>MESRVTPVAVIGMGCRLPGGINSPDKLWESLLRGDDLVTEIPPDRWDADDYYDPEPGVPGRSVSRWGGFLDDVAGFDAEFFGISEREATSIDPQQRLLLETSWEAIEHAGLDPASLAGSSTAVFTGLTHEDYLVLTTTAGGLASPYVVTGLNNSVASGRIAHTLGLHGPAMTFDTACSSGLMAVHLACRSLHDGEADLALAGGCAVLLEPHASVAASAQGMLSSTGRCHSFDADADGFVRSEGCAMVLLKRLPDALRDGNRIFAVVRGTATNQDGRTETLTMPSEDAQVAVYRAALAAAGVQPETVGVVEAHGTGTPIGDPIEYRSLARVYGAGTPCALGSAKSNMGHSTASAGTVGLIKAILSLRHGVVPPLLHFNRLPDELSDVETGLFVPQAVTPWPNGNDHTPKRVAVSSFGMSGTNVHAIVEEAPAEASAPESSPGDAEVGPRLFMLSSTSSDALRQTARQLATWVEEHQDCVAASDLAYTLARGRAHRPVRTAVVAANLPELVEGLREVADGDALYDAAVGHGDRGPVWVFSGQGSQWAAMGTQLLASEPVFAATIAKLEPVIAAESGFSVTEAITAQQTVTGIDKVQPAVFAVQVALAATMEQTYGVRPGAVVGHSMGESAAAVVAGALSLEDAARVICRRSKLMTRIAGAGAMGSVELPAKQVNSELMARGIDDVVVSVVASPQSTVIGGTSDTVRDLIARWEQRDVMAREVAVDVASHSPQVDPILDDLAAALADIAPMTPKVPYYSATLFDPREQPVCDGAYWVDNLRNTVQFAAAVQAAMEDGYRVFAELSPHPLLTHAVEQTGRSLDMSVAALAGMRREQPLPHGLRGLLTELHRAGAALDYSALYPAGRLVDAPLPAWTHARLFIDDDGQEQRAQGACTITVHPLLGSHVRLTEEPERHVWQGDVGTSVLSWLSDHQVHNVAALPGAAYCEMALAAAAEVFGEAAEVRDITFEQMLLLDEQTPIDAVASIDAPGVVNFTVETNRDGETTRHATAALRAAEDDCPPPGYDITALLQAHPHAVNGTAMRESFAERGVTLGAAFGGLTTAHTAEAGAATVLAEVALPASIRFQQGAYRIHPALLDACFQSVGAGVQAGTATGGLLLPLGVRSLRAYGPTRNARYCYTRLTKAFNDGTRGGEADLDVLDEHGTVLLAVRGLRMGTGTSERDERDRLVSERLLTLGWQQRALPEVGDGEAGSWLLIDTSNAVDTPDMLASTLTDALKSHGPQGTECASLSWSVQDTPPNDQAGLEKLGSQLRGRDGVVIVYGPRVGDPDEHSLLAGREQVRHLVRITRELAEFEGELPRLFVVTRQAQIVKPHDSGERANLEQAGLRGLLRVISSEHPMLRTTLIDVDEHTDVERVAQQLLSGSEEDETAWRNGDWYVARLTPSPLGHEERRTAVLDPDHDGMRVQVRRPGDLQTLEFVASDRVPPGPGQIEVAVSMSSINFADVLIAFGRFPIIDDREPQLGMDFVGVVTAVGEGVTGHQVGDRVGGFSEGGCWRTFLTCDANLAVTLPPGLTDEQAITAATAHATAWYGLNDLAQIKAGDKVLIHSATGGVGQAAISIARAKGAEIFATAGNPAKRAMLRDMGVEHVYDSRSVEFAEQIRRDTDGYGVDIVLNSLTGAAQRAGLELLAFGGRFVEIGKADVYGNTRLGLFPFRRGLTFYYLDLALMSVTQPDRVRELLATVFKLTADGVLTAPQCTHYPLAEAADAIRAMSNAEHTGKLVLDVPRSGRRSVAVTPEQAPLYRRDGSYIITGGLGGLGLFFASKLAAAGCGRIVLTARSQPNPKARQTIEGLRAAGADIVVECGNIAEPDTADRLVSAATATGLPLRGVLHSAAVVEDATLTNITDELIDRDWSPKVFGSWNLHRATLGQPLDWFCLFSSGAALLGSPGQGAYAAANSWVDVFAHWRRAQGLPVSAIAWGAWGEVGRATFLAEGGEIMITPEEGAYAFETLVRHDRAYSGYIPILGAPWLADLVRRSPWGEMFASTGQRSRGPSKFRMELLSLPQDEWAGRLRRLLVEQASVILRRTIDADRSFIEYGLDSLGMLEMRTHVETETGIRLTPKVIATNNTARALAQYLADTLAEEQAAAPAASKLAAALEHHHHHH[3x]

As exemplified by isoniazid, which targets the enoylreductase in mycolic acid biosynthesis, mycocerosic acid synthase (MAS) offers a potential drug target by producing part of phthiocerol dimycocerosate (PDIM), a key component of the cell envelope. MAS, a fully reducing iterative type I polyketide synthase (PKS), is composed of six domains that together catalyze the elongation of n-C6-C20 fatty acids to prepare mycocerosic acid. Using a combination of dual covalent crosslinking and cryo-EM analyses, we elucidate the structure of mycocerosic acid synthase from Mycobacterium tuberculosis trapped in two distinct catalytic states during its iterative cycle. These structures reveal domain architecture of the acyl carrier protein mediating condensation and dehydration through dual site-selective crosslinking of the acyl carrier protein with the ketosynthase and dehydratase domains.

We also obtained a density map for complex B from the same dataset with a higher overall resolution (3.22 Å) that further elucidates details of the condensation compartment (KS-LD-AT), with only one ACP crosslinked at KS. Complex B revealed the homodimeric condensation compartment (KS-LD-AT) with one ACP crosslinked at KS via 1, while the other KS was inhibited by 1 in small molecule form (without ACP). Covalent bond S-C between the KS active site Cys177 and the reactive α-position of the crosslinker, as well as the O-P covalent bond between the ACP active residue Ser2060 and the PPant arm, were determined by continuous map density. Interactions between ACP and KS are limited to a single hydrogen bond between Arg2045 on loop 1 of the ACP and Glu79 of KS along with weak hydrophobic and electrostatic interactions. Complex B reveals that the docking of ACP on KS is mainly facilitated by interactions with the neighboring AT domain via hydrogen bonding between Arg2032 and Arg2033 on helix 1 and Arg2090 on helix 4 with Asp819 on the AT domain. In MAS complex B, the crosslinker, tethered through a phosphodiester linkage to Ser2060 of ACP, has the PPant arm forming hydrogen bonds with residues Thr279 and Thr281 in KS. The warhead carbonyl of crosslinker 1 coordinates with two highly conserved residues His312 and His348, trapping the transacylation (substrate loading or reloading) state of KS in its gate-closed form. Supported by continuous map density, the C16 acyl tail of 1 is buried deep within the hydrophobic tunnel formed by the KS • KS’ dimeric interface. In terms of substrate chain length, it is noteworthy that the two substrate tunnels formed by the KS • KS’ dimer in complex B are connected, contributing to a potential substrate tunnel sharing to accommodate C22-C28 mycocerosic acids products. In complex B, MAS potentially adopts KS gating loops similar to E. coli type II KSs, and the presence of key gating residues is essential for activity.>MATKSVLMLGSGFVTRPTLDVLTDSGIKVTVACRTLESAKKLSAGVQHSTPISLDVNDDAALDAEVAKHDLVISLIPYTFHATVIKSAIRQKKHVVTTSYVSPAMMELDQAAKDAGITVMNEIGLDPGIDHLYAIKTIEEVHAAGGKIKTFLSYCGGLPAPESSDNPLGYKFSWSSRGVLLALRNAASFYKDGKVTNVAGPELMATAKPYFIYPGFAFVAYPNRDSTPYKERYQIPEADNIVRGTLRYQGFPQFIKVLVDIGFLSDEEQPFLKEAIPWKEATQKIVKASSASEQDIVSTIVSNATFESTEEQKRIVAGLKWLGIFSDKKITPRGNALDTLCATLEEKMQFEEGERDLVMLQHKFEIENK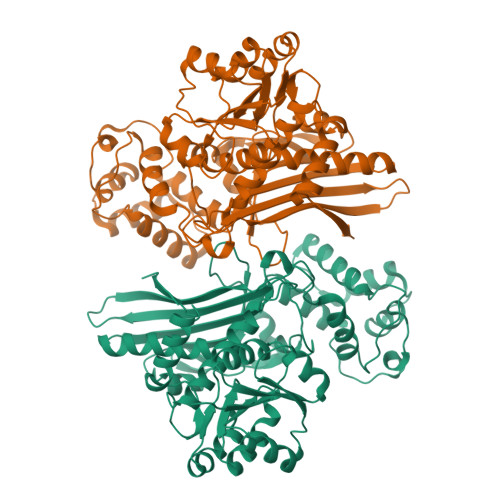DGSRETRTSSLCEYGAPIGSGGYSAMAKLVGVPCAVAVKFVLDGTISDRGVLAPMNSKINDPLMKELKEKYGIECKEKVVA[2x]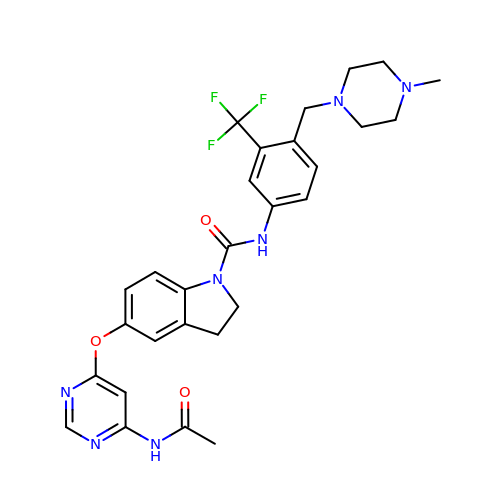5-{[6-(acetylamino)pyrimidin-4-yl]oxy}-N-{4-[(4-methylpiperazin-1-yl)methyl]-3-(trifluoromethyl)phenyl}-2,3-dihydro-1H-indole-1-carboxamide | C28 H30 F3 N7 O3 | VQLNKQZLPGLOSI-UHFFFAOYSA-N> MANKAVNDFILAMNYDKKKLLTHQGESIENRFIKEGNQLPDEFVVIERKKRSLSTNTSDISVTATNDSRLYPGALLVVDETLLENNPTLLAVDRAPMTYSIDLPGLASSDSFLQVEDPSNSSVRGAVNDLLAKWHQDYGQVNNVPARMQYEKITAHSMEQLKVKFGSDFEKAANSLDIDFNAVHSGEKQIQIVNFKQIYYTVSVDAVKNPGDVFQDTVTVEDLKQRGISAERPLVYISSVAYGRQVYLKLETTSKSDEVQAAFEAAILGVKVAPQTQWKQILDNTEVKAVILGGDPSSGARVVTGKVDMVEDLIQEGSRFTADHPGLPISYTTSFLRDNVVATFQNSTDYVETKVTAYRNGDLLLDHSGAYVAQYYITWDELSYDHQGKEVLTPKAWDRNGQDLTAHFTTSIPLKGNVRNLSVKIRECTGLAWEWWRTVYEKTDLPLVRKRTISIWGTTLYPQVEDKVEND

Gram-positive bacteria, including the common wound-infecting Staphylococcus aureus, the virulent food-borne pathogen Listeria monocytogenes, and Streptococcus pneumoniae that causes pneumonia, utilize cholesterol-dependent cytolysins (CDCs) to attack and kill mammalian and human cells. The bacteria produce and release CDCs as water-soluble monomers that attach to cholesterol-containing cell membranes, where they assemble into large, 200–500 Å cytolytic pores. X-ray structures of pneumolysin (PLY) from S. pneumoniae show that the soluble toxin monomers are roughly rod-shaped and consist of four domains (D1-D4). Sequence comparison suggests that all CDCs have the same domain structure and therefore insert into target membranes in essentially the same way.

We determined the structure of the ring-shaped ~2.2 MDa PLY pore complex by cryoEM. Pore complexes were rings of 42 subunits with an aggregate molecular mass of 2.2 MDa. In total, 6461 ring images were combined to generate a 3D map with 42-fold symmetry at 4.5 Å resolution (Figure 1—figure supplements 2B and 3,). Comparison to the soluble form revealed a complete reorganization of the toxin upon membrane insertion. Of the four protein domains D1-D4 in the x-ray structure, D1 and D4 fitted the map of the pore complex with minimal modifications (Figure 2—figure supplements 1–3). The elongated two-stranded β-sheet of D2 rotates from its vertical position in the x-ray structure by 90° around a short glycine linker to an orientation parallel to the membrane plane in the pore complex. D2 connects D1 to D4, and its rotation results in a roughly linear translation of D1 by 35 Å towards the membrane surface and by 30 Å towards the pore centre. In the pore complex, both bundles refold into four 85 Å β-strands, which form two parallel β-hairpins that insert into and traverse the lipid bilayer. The β-hairpins of neighbouring subunits coalesce into one extensive, 168-strand β-barrel with an inner diameter of 260 Å. In the ring, the HTH motifs of the 42 subunits line up in one plane on the exoplasmic side of the molecule and form an α-barrel inside the β-barrel, restricting the pore diameter locally to 250 Å.>[3x]MRCIGISNRDFVEGVSGGSWVDIVLEHGSCVTTMAKNKPTLDFELIKTEAKQPATLRKYCIEAKLTNTTTESRCPTQGEPTLNEEQDKRFVCKHSMVDRGWGNGCGLFGKGGIVTCAMFTCKKNMEGKIVQPENLEYTVVIT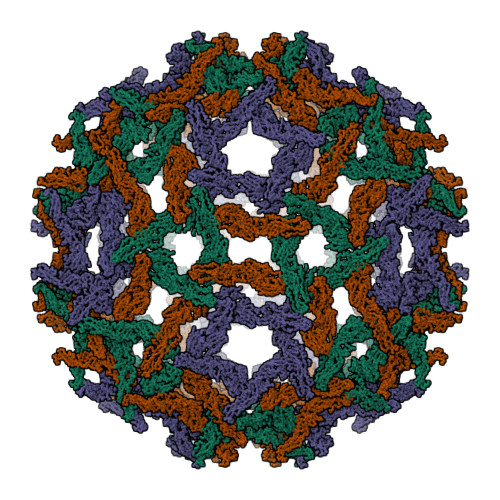PHSGEEHAVGNDTGKHGKEVKITPQSSITEAELTGYGTVTMECSPRTGLDFNEMVLLQMKDKAWLVHRQWFLDLPLPWLPGADTQGSNWIQKETLVTFKNPHAKKQDVVVLGSQEGAMHTALTGATEIQMSSGNLLFTGHLKCRLRMDKLQLKGMSYSMCTGKFKVVKEIAETQHGTIVIRVQYEGDGSPCKIPFEIMDLEKRHVLGRLITVNPIVTEKDSPVNIEAEPPFGDSYIIIGVEPGQLKLNWFKKG>[2x]EQARPADDALAALGAQLFVDPALSRNATQSCATCHDPARAFTDPREGKAGLAVSVGDDGQSHGDRNTPTLGYAALVPAFHRDANGKYKGGQFWDGRADDLKQQAGQPMLNPVQMAMPDRAAVAARLRDDPAYRTGFEALFGKGVLDDPERAFDAAAEALAAYQATGEFSPFDSKYDRVMRGEEKFTPLEEFGYTVFITWNCRLCHMQRKQGVAERETFTNFEYHNIGLPVNETAREASGLGADHVDHGLLARPGIEDPAQSGRFKVPSLRNVAVTGPYMHNGVFTDLRTAILFYNKYTSRRPEAK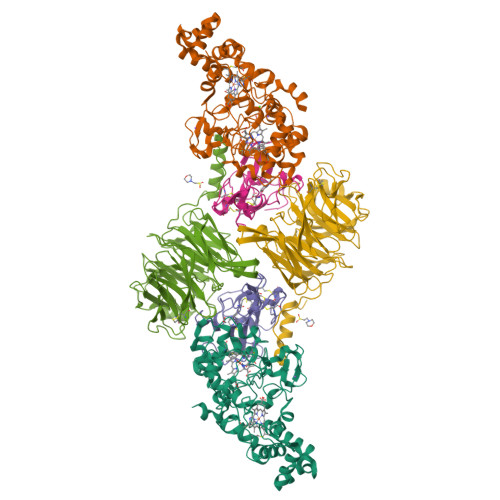INPETGAPWGEPEVARNLSLAELQSGLMLDDGRVDALVAFLETLTDRRYEPLLEESRAAQKDHHHHHH;>ADAPAGTDPRAKWVPQDNDIQACDYWRHCSIDGNICDCSGGSLTNCPPGTKLATASWVASCYNPTDGQSYLIAYRDCCGYNVSGRCPCLNTEGELPVYRPEFANDIIWCFGAEDDAMTYHCTISPIVGKASHHHHHH[2x];>[2x]DAPEAETQAQETQGQAAARAAAADLAAGQDDEPRILEAPAPDARRVYVNDPAHFAAVTQQFVIDGEAGRVIGMIDGGFLPNPVVADDGSFIAHASTVFSRIARGERTDYVEVFDPVTLLPTADIELPDAPRFLVGTYPWMTSLTPDGKTLLFYQFSPAPAVGVVDLEGKAFKRMLDVPDCYHIFPTAPDTFFMHCRDGSLAKVAFGTEGTPEITHTEVFHPEDEFLINHPAYSQKAGRLVWPTYTGKIHQIDLSSGDAKFLPAVEALTEAERADGWRPGGWQQVAYHRALDRIYLLVDQRDEWRHKTASRFVVVLDAKTGERLAKFEMGHEIDSINVSQDEKPLLYALSTGDKTLYIHDAESGEELRSVNQLGHGPQVITTADMG The helical morphology of Campylobacter jejuni, a bacterium involved in host gut colonization and pathogenesis in humans, is determined by the structure of the peptidoglycan (PG) layer. Pgp2 is an LD-carboxypeptidase that cleaves D-Ala from both monomeric and cross-linked tetrapeptides. The structure of Pgp2 contains an N-terminal helix (residues Q43-I51), the catalytic LD-CPase domain (residues V65-K201), and the C-terminal NTF2 domain (residues K208-Q325), each connected to the next domain by a single loop. In summary, we show that helical shape in C. jejuni depends on both the LD-CPase and NTF2 domains of Pgp2.

A recombinant Pgp2 construct (Pgp243-325) containing residues 43–325 of the native sequence (cjj81176_0915) is enzymatically active and was suitable for structural characterization. The Pgp2 structure contains one Pgp2 molecule in the asymmetric unit. An extensive interface with a buried surface area of 1130 Å2 is found between the LD-CPase and NTF2 domains, as calculated by the PISA server. The likely catalytic triad (C174-H157-G158) is located on the central stands β5–β6. The NTF2 domain contains three helices (α6–α8) wrapped around a curved antiparallel β-sheet (β8–β11), which together forms a cone shape domain with a broad pocket. Regions of high sequence conservation are observed on one side of the molecule, focused in two clusters. The first cluster is in proximity to the catalytic triad in the LD-CPase domain. The second cluster is formed by 17 primarily aromatic (41%) and charged (30%) residues that are clustered in the pocket of the NTF2 domain. In the wild-type Pgp2 crystal structure, the average B-factor of β9-β10 (residues 292–310) was 53.4 Å2, 1.8-fold higher than the average B-factor over all residues. The conserved CPase active site and NTF2 domain pocket are ∼40 Å apart along the same side of the protein surface.

> GSHMQKDFWLSEIGDKNISLGYYDDNVAIVLTNKTDKILRVYSYEDGKIRKDFEQKEIITGLMGDKKIEGDLKTPVGFYELGRKFNPGDPYYGPFAFATTYPNLLDKVQGKTGGGIWIHGYPLDGSRLDEFKTRGCIALFNNNLEKFAQVVQDKKVFVMTEEKEKIRAKKDQIASLLADLFTWKLAWTNSDTNTYLSFYDEQEFKRFDKMKFEQFASMKKSIFSRKEDKKIKFSDINISPYPNLENETMYRISFYEDYYTKNYQFRGDKILYVKIDSKGKMKILAEQ> QDNSRYTHFLTQHYDAKPQGRDDRYCESIMRRRGLTSPCKDINTFIHGNKRSIKAICENKNGNPHRENLRISKSSFQVTTCKLHGGSPWPPCQYRAT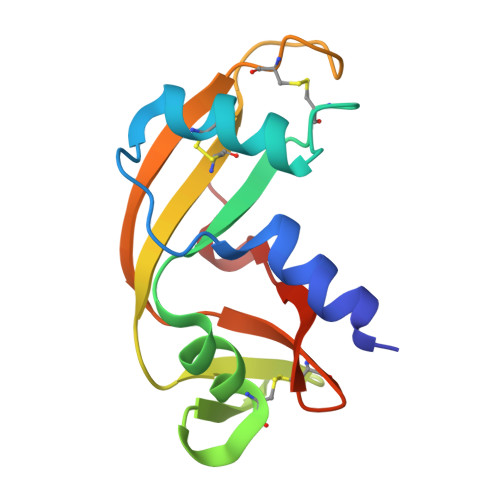AGFRNVVVACENGLPVHLDQSIFRRP> MRGSHHHHHHTDLRADKASSIELKFDRNKGEVGDILIGTVRINNIKNFAGFQVNIVYDPKVLMAVDPETGKEFTSSTFPPGRTVLKNNAYGPIQIADNDPEKGILNFALAYSYIAGYKETGVAEESGIIAKIGFKILQKKSTAVKFQDTLSMPGAISGTQLFDWDGEVITGYEVIQPDVLSLGDEP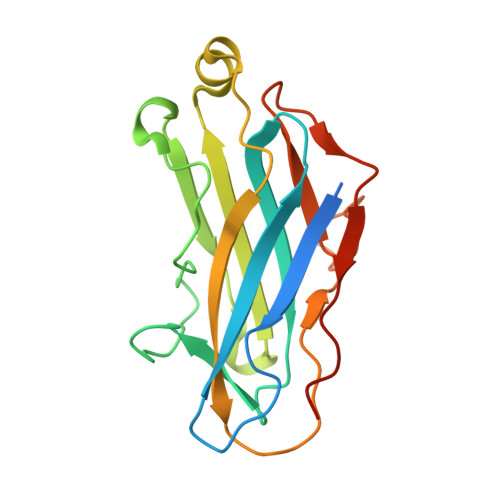Y>MKTIGLLGGMSWESTIPYYRLINEGIKQRLGGLHSAQVLLHSVDFHEIEECQRRGEWDKTGDILAEAALGLQRAGAEGIVLCTNTMHKVADAIESRCTLPFLHIADATGRAITGAGMTRVALLGTRYTMEQDFYRGRLTEQFSINCLIPEADERAKINQIIFEELCLGQFTEASRAYYAQVIARLAEQGAQGVIF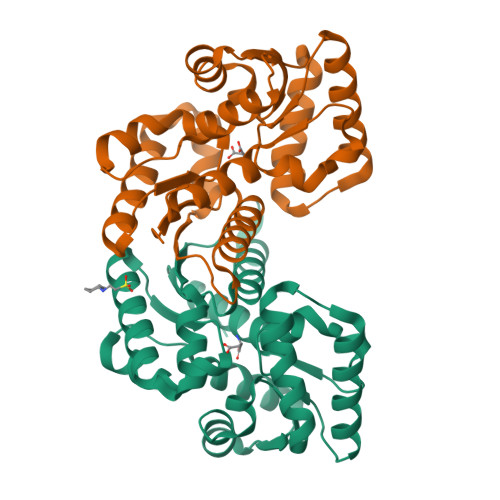GCTEIGLLVPEERSVLPVFDTAAIHAEDAVAFMLSLEHHH[2x]> UGCXCCUAGUAC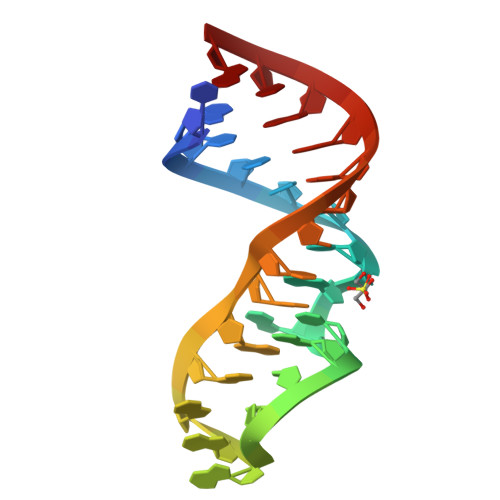GAGAGGACCGGAGUG>[4x]GPLGSPEFPGGAFRTQKPSLNTVNVVGSSMGSGGVFTIDGKIKCVTAAHVLTGNSARVSGVGFNQMLDFDVKGDFAIADCPNWQGVAPKAQFCED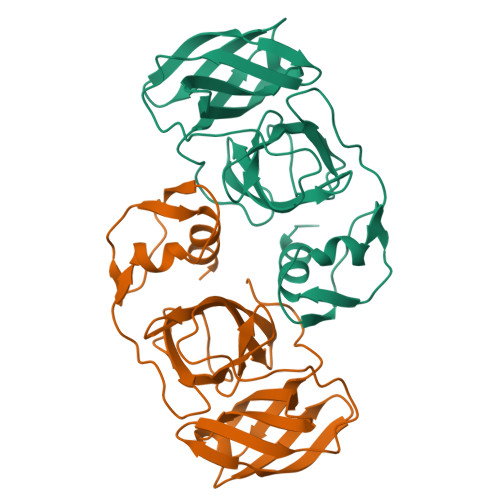GWTGRAYWLTSSGVEPGVIGNGFAFCFTACGDSGSPVITEAGELVGVHTGSNKQGGGIVTRPSGQFCNVKPIKLSELSEFFAGPKVPLGDVKIGSHIIKDTCEVPSDLCALLAAKPELE> EDDLYRQSLEIISRYLREQATGSKDSKPLGEAG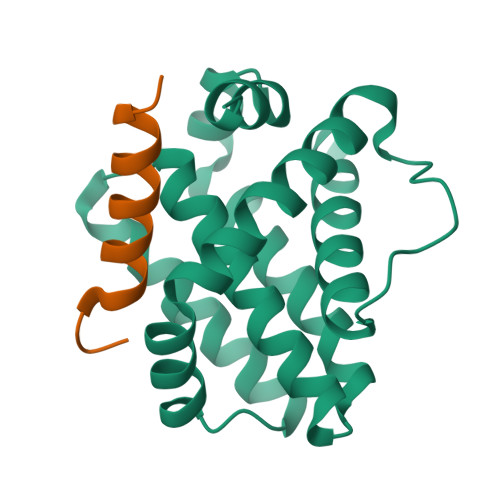AAGRRALETLRRVGDGVQRNHETAFQGMLRKLDIKNEDDVKSLSRVMIHVFSDGVTNWGRIVTLISFGAFVAKHLKTINQESCIEPLAESITDVLVRTKRDWLVKQRGWDGFVEFFHVEDLEGG;> PADLKDECAQLRRIGDKVNLRQKLLN> MASLPKRIIKETEKLVSDPVPGITAEPHDDNLRYFQVTIEGPEQSPYEDGIFELELYLPDDYPMEAPKVRFLTKIYHPAIDRLGRISLDVLKTNWSPALQIRTVLLSIQALLASPNPNDPLANDV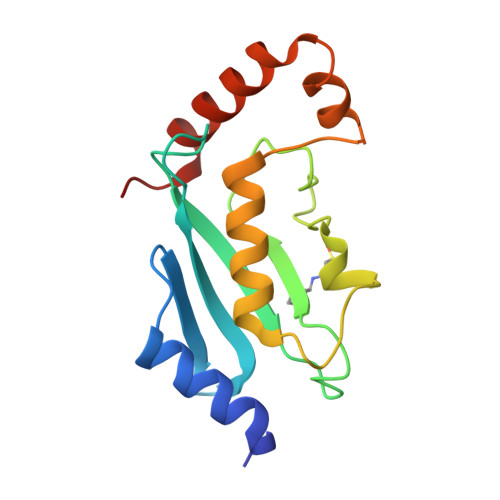AEDWIKNEQGAKAKAREWTKLYAKKKPE>SNAIEEVYEATLDAIQGALNCDRASILLFDEAGTMRFVAARGLSEHYQRAVDGHSPWITGANEPEPIFVENVDDAEFSRELKESIVGEGIAALGFFPLVTEGRLIGKFMTYYDRPHRFADSEIGMALTIA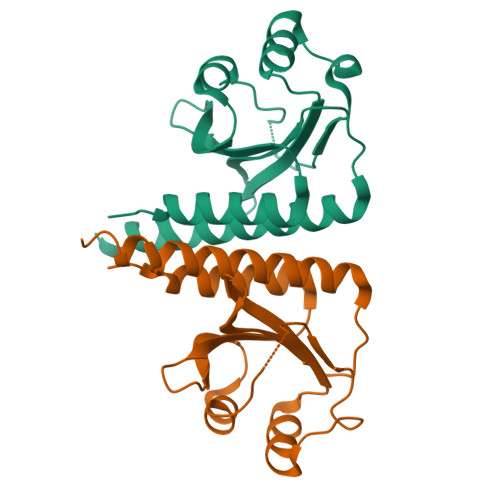RQLGFSIQRMRAEYARRQAEE[2x]> MNVYDDVLDATVVSHSLATHFTTSDYEELLVVRTNILSVYRPTRDGKLYLTDEFKFHGLITDIGLIPQKDSPLSCLLLCTGVAKISILKFNTLTNSIDTLSLHYYEGKFKGKSLVELAKISTLRMDPGSSCALLFNNDIIAFLPFHVNKNDDDEEEEDEDENIDDSELIHSMNQKSQGTNTFNKRKRTKLGDKFTAPSVVLVASELYEGAKNIIDIQFLKNFTKPTIALLYQPKLVWAGNTTISKLPTQYVILTLNIQPAESATKIESTTIAFVKELPWDLHTIVPVSNGAIIVGTNELAFLDNTGVLQSTVLLNSFADKELQKTKIINNSSLEIMFREKNTTSIWIPSSKSKNGGSNNDETLLLMDLKSNIYYIQMEAEGRLLIKFDIFKLPIVNDLLKENSNPKCITRLNATNSNKNMDLFIGFGSGNALVLRLNNLKSTIETREAHNPSSGTNSLMDINDDDDEEMDDLYADEAPENGLTTNDSKGTVETVQPFDIELLSSLRNVGPITSLTVGKVSSIDDVVKGLPNPNKNEYSLVATSGNGSGSHLTVIQTSVQPEIELALKFISITQIWNLKIKGRDRYLITTDSTKSRSDIYESDNNFKLHKGGRLRRDATTVYISMFGEEKRIIQVTTNHLYLYDTHFRRLTTIKFDYEVIHVSVMDPYILVTVSRGDIKIFELEEKNKRKLLKVDLPEILNEMVITSGLILKSNMCNEFLIGLSKSQEEQLLFTFVTADNQIIFFTKDHNDRIFQLNGVDQLNESLYISTYQLGDEIVPDPSIKQVMINKLGHDNKEEYLTILTFGGEIYQYRKLPQRRSRFYRNVTRNDLAITGAPDNAYAKGVSSIERIMHYFPDYNGYSVIFVTGSVPYILIKEDDSTPKIFKFGNIPLVSVTPWSERSVMCVDDIKNARVYTLTTDNMYYGNKLPLKQIKISNVLDDYKTLQKLVYHERAQLFLVSYCKRVPYEALGEDGEKVIGYDENVPHAEGFQSGILLINPKSWKVIDKIDFPKNSVVNEMRSSMIQINSKTKRKREYIIAGVANATTEDTPPTGAFHIYDVIEVVPEPGKPDTNYKLKEIFQEEVSGTVSTVCEVSGRFMISQSQKVLVRDIQEDNSVIPVAFLDIPVFVTDSKSFGNLLIIGDAMQGFQFIGFDAEPYRMISLGRSMSKFQTMSLEFLVNGGDMYFAATDADRNVHVLKYAPDEPNSLSGQRLVHCSSFTLHSTNSCMMLLPRNEEFGSPQVPSFQNVGGQVDGSVFKIVPLSEEKYRRLYVIQQQIIDRELQLGGLNPRMERLANDFYQMGHSMRPMLDFNVIRRFCGLAIDRRKSIAQKAGRHAHFEAWRDIINIEFSMRSLCQGK;> PSLIHPDTAKYPFKFEPFLRQEYSFSLDPDRPICEFYNSREGPKSCPRGPLCPKKHVLPIFQNKIVCRHWLRGLCKKNDQCEYLHEYNLRKMPECVFFSKNGYCTQSPDCQYLHIDPASKIPKCENYEMGFCPLGSSCPRRHIKKVFCQRYMTGFCPLGKDECDMEHPQFIIPDEGSKLRIKRDDEINTRKMDEEKERRLNAIINGEV;> MDGHNQNQYQNQNQIQQSQQPPLKKYVTQRRSVDVSSPYINLYYNRRHGLPNLVVEPETSYTIDIMPPNAYRGRDRVINLPSKFTHLSSNKVKHVIPAIQWTPEGRRLVVATYSGEFSLWNASSFTFETLMQAHDSAVTTMKYSHDSDWMISGDADGMIKIWQPNFSMVKEIDAAHTESIRDMAFSSNDSKFVTCSDDNILKIWNFSNGKQERVLSGHHWDVKSCDWHPEMGLIASASKDNLVKLWDPRSGNCISSILKFKHTVLKTRFQPTKGNLLMAISKDKSCRVFDIRYSMKELMCVRDETDYMTLEWHPINESMFTLACYDGSLKHFDLLQNLNEPILTIPYAHDKCITSLSYNPVGHIFATAAKDRTIRFWTRARPIDPNAYDDPTYNNKKINGWFFGINNDINAVREKSEFGAAPPPPATLEPHALPNMNGFINKKPRQEIPGIDSNIKSSTLPGLSIXXXXX

The 3′-end processing machinery includes the highly conserved cleavage and polyadenylation factor (CPF in yeast, CPSF in metazoans). CPF interacts with Pol II during transcription, monitoring the nascent pre-mRNA until it recognizes specific RNA elements. It is reported to contain 15 different subunits, including the Ysh1/CPSF73 endonuclease that cleaves the pre-mRNA, the Pap1/PAP polymerase that adds the polyadenylate [poly(A)] tail, and two protein phosphatases (Ssu72/SSU72 and Glc7/PP1) that regulate transcription and 3′-end processing (1–7). Computational analysis revealed a protein–protein interaction network in which subunits are organized into three prominent modules centered around the CPF enzymatic activities: nuclease ( Ysh1), phosphatase (Ssu72, Glc7), and polymerase (Pap1). The poly(A) polymerase module contains five subunits: Cft1, Pfs2, Pap1, Fip1, and Yth1.

Next, because of the central role of polyadenylation in 3′-end processing, we developed a strategy to overexpress the polymerase module in insect cells for structural and biochemical characterization. In our cryo-EM map, three of the four subunits are well ordered: Cft1 (residues 1 to 1357), Pfs2 (residues 27 to 411), and Yth1 (residues 1 to 94). Cft1 forms the core of the complex and is composed of three seven-bladed β propellers followed by a C-terminal helical domain. β propeller 1 (BP1) and BP2 are each formed of contiguous sequences. The C-terminal helical domain of Cft1 is located at the nexus of the three β propellers, further stabilizing the fold. Our structure reveals an extensive interface between Cft1 and Pfs2, burying >4200 Å2 surface area. Almost 50 amino acids in the N-terminal region of Pfs2 are inserted into the cavity between Cft1-BP1 and -BP3, forming contacts with the tops of both β propellers. Yth1 is anchored onto the complex by an extended N-terminal segment that binds in the central cavity of Cft1-BP3 and continues across a hydrophobic external face. Next, two of the five Cys-Cys-Cys-His (CCCH) zinc fingers pack into the interface between Cft1 and Pfs2. The cryo-EM structure of the Cft1–Pfs2–Yth1 complex of the polymerase module has a markedly similar architecture to the eukaryotic DDB1- DDB2 and SF3b complexes.>GSLRPLSEVNQHSQLMAQLVEVIEDSFQMKVNKESVNYLRLIRHIRFTIERIKKEEPTKEPEKLMLLLKNEYPLCYNTAWKLIKILQQTLKKPVHEAEAVYL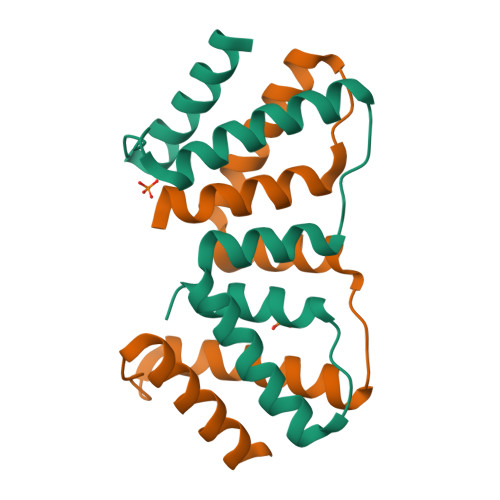TLHLIPINQ[2x]> MSDWSLSQLFASLHEDIQLRLGTARKAFQHPGAKGDASEGVWIEMLDTYLPKRYQAANAFVVDSLGNFSDQIDVVVFDRQYSPFIFKFNEQIIVPAESVYAVFEAKQSASADLVAYAQRKVASVRRLHRTSLPIPHAGGTYPAKPLIPILGGLLTFESDWSPALGM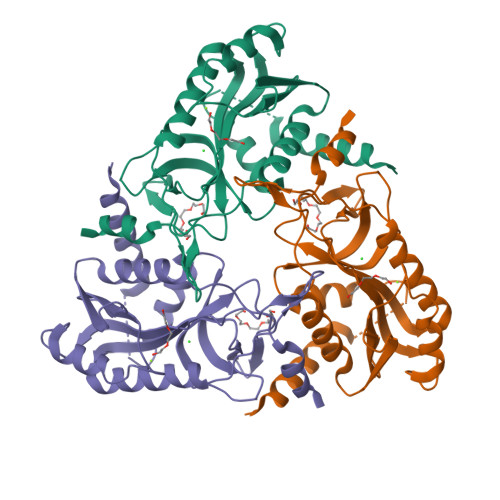SFDKALNGDLSDGRLDMGCVASHGHFYFNNIDSKFNFEHGNKPATAFLFRLIAQLQFSGTVPMIDIDAYGKWLAN Diadenosine-5′,5-P1,P4-tetraphosphate (Ap4A) is a ubiquitous second messenger from bacteria to higher eukaryotes, which responds to environmental stresses and cell cycle phases. Ap4A then binds to the histidine triad nucleotide-binding protein 1 (HINT1), thereby disrupting the protein–protein interaction with microphthalmia-associated transcription factor (MITF), and the released MITF eventually promotes the transcription of mast cell activation genes. The HINT1 protein is a compact and symmetric dimer, with two adenosine pockets at opposite sides. Here we report that Ap4A specifically polymerizes HINT1 into (HINT1-Ap4A)n (HAn) filaments in solution and in the activated RBL cells.

We then made an H114A mutant to inactivate the hydrolysis activity of HINT1. Finally, to reveal the molecular specificity of Ap4A to induce HAn, we further solved the co-crystal structures of HINT1H114A-ATP and HINT1H114A-Ap3A. Only the AMP portion of these molecules were resolved in the adenosine pockets of HINT1, with the remaining atoms of ATP or Ap3A untraceable. Neither ATP (with only one adenosine moiety) nor Ap3A (with a shorter phosphodiester linkage) could recruit HINT1 dimers to form polymer in solution. Our results show that Ap3A, Ap5A, AMP, and ATP could not induce HINT1 polymerization. The five-phosphate linkage in Ap5A adopted a bent and zigzag conformation compared with the straight conformation of Ap4A, suggesting that the increased length of Ap5A is too long to stabilize the HAn interface as Ap4A does. Together, these results indicate that the bivalent characteristic, the length of the phosphodiester linkage, and the interaction of phosphates of Ap4A with HINT1 were all critical for HAn formation.

>SLMADEIAKAQVARPGGDTIFGKIIRKEIPAKIIFEDDRCLAFHDISPQAPTHFLVIPKKHISQISVAEDDDESLLGHLMIVGKKCAADLGLNKGYRMVVNEGSDGGQSVYHVHLAVLGGRQMHWPPG[4x]> MLAKRIIACLDVKDGR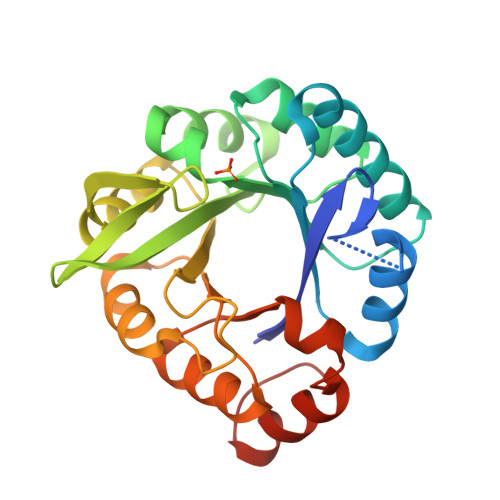VVKGSNFENLRDSGDPVELGKFYSEIGIDELVFLDITASVEKRKTMLELVEKVAEQIDIPFTVGGGIHDFETASELILRGADKVSINTAAVENPSLITQIAQTFGSQAVVVAIDAKRVDGEFMVFTYSGKKNTGILLRDWVVEVEKRGAGEILLTSIDRDGTKSGADTEMIRFVRPLTTLPIIASGGAGKMEHFLEAFLAGADAALAASVFHFREIDVRELKEYLKKHGVNVRLEGL> TVIMREAARHGLTIVRLQPQGSRLSLTVQPAD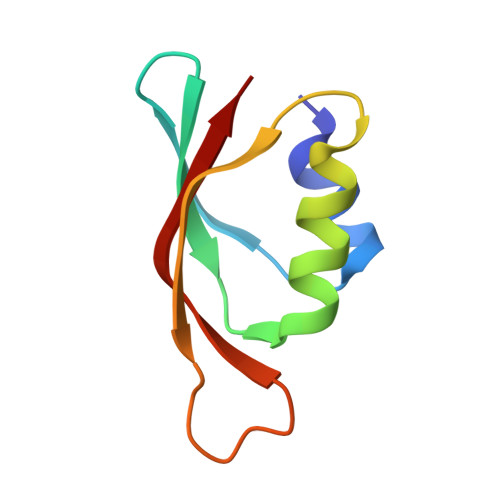FQALMAWLDALGQAGMTTATLAVTAVAQQPGWVTVNTLVLER Here, the current status of the fully automated ambient-temperature beamline VMXi at Diamond Light Source is described, and a highly efficient pipeline from protein sample to final multi-crystal data analysis and structure determination is shown. The VMXi beamline and its associated PXF within the Research Complex at Harwell offer a highly automated pipeline where researchers provide a suitable protein sample that is used for robotic crystallization, monitoring and subsequent in situ data collection from crystals in crystallization plates or in thin-film sample delivery systems. Here we present illustrative examples of data measured using VMXi from a variety of proteins comprising both conventional crystallographic standards and ‘real world’ user samples. Routine RT data collection provides a useful capability that is highly relevant to studying protein dynamics and ligand binding without the complication of cryo-cooling.

Other users tend to focus on groups of proteins with homologous functions from a range of microorganisms. This is the case of a group working with cytochromes c′. Furthermore, they pose a challenge as their heme centre is very sensitive to radiation, and thus careful data collection and analysis are crucial. A second cytochrome c′ protein from T. thermophilus (TTCP), in this case with β-sheet fold, presented a greater challenge. Firstly, crystals grow in clusters of stacked plates [Fig. 2(f)], making it impracticable to harvest and cryo-cool without further optimization of crystallization conditions, but the ability to collect data in situ at VMXi made it possible to carefully select positions for data collection around the edges of the cluster [Fig. 2(f)] and the microfocus beam allowed useful datasets to be measured. A full comparison between the RT and 100 K structures was not feasible because the crystallization conditions as well as space group differed.

> GLPYPEGYRFWTHVKSMELKPGHPLYESFGGLHHIYVNPTGLRTYLEGKKAPFPKGTVIVFDLLEAKVEGNALLEGPRKLIGVMAKDPGRYPDTGGWGYYAFGPDKKPLAIDPKACHACHQGAANTDYVFSAFRP> GPAFEFAVAMMKRNSSTVKTEYGEFTMLGIYDKWAVLPRHAKPGPTILMNDQEVSVLDAKELVDKDGTNLELTLLKLNRNEKFRDIRGFLAKEEVEVNEAVLAINTSKFPNMY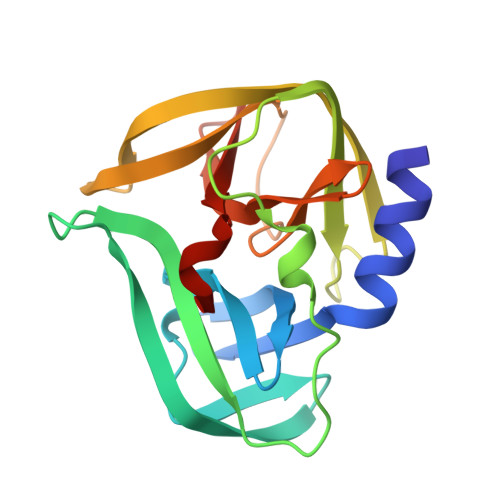IPVGQVTDYGFLNLGGTPTKRMLMYNFPTRAGQCGGVLMSTGKVLGIHVGGNGHQGFSAALLKHYFNDEQ> GSPNSPATGEKKECWSWESYLEEQKAITAPVSLFQDSQAVTHNKNGFKLGMKLEGIDPQHPSMYFILTVAEVCGYRLRLHFDGYSECHDFWVNANSPDIHPAGWFEKTGHKLQPPKGYKEEEFSWSQYLRSTRAQAAPKHLFVSQSHSPPPLGFQVGMKLEAVDRMNPSLVCVASVTDVVDSRFLVHFDNWDDTYDYWCDPSSPYIHPVGWCQKQGKPLTPPQDYPDPDNFCWEKYLEETGASAVPTWAFKVRPPHSFLVNMKLEAVDRRNPALIRVA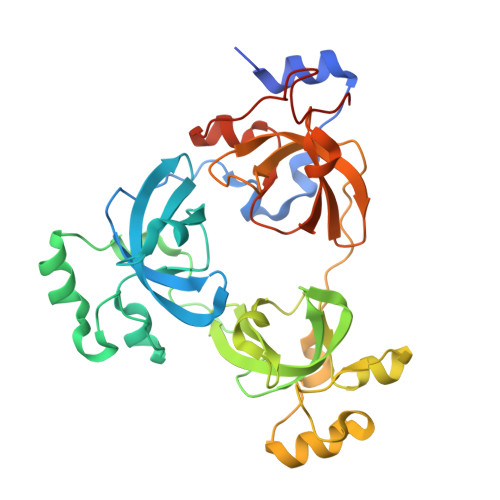SVEDVEDHRIKIHFDGWSHGYDFWIDADHPDIHPAGWCSKTGHPLQPPLGPREPSSAVDSSGRIVTD>IPCGESCVWLPCISSAIGCSCKSKV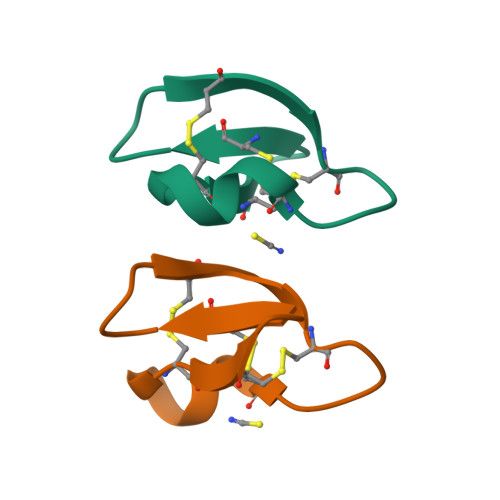CYRNG[2x]> LLEAIAIALTAAHFGAPLLYYWRAKRWLKKPWDVAPDPTYRPRV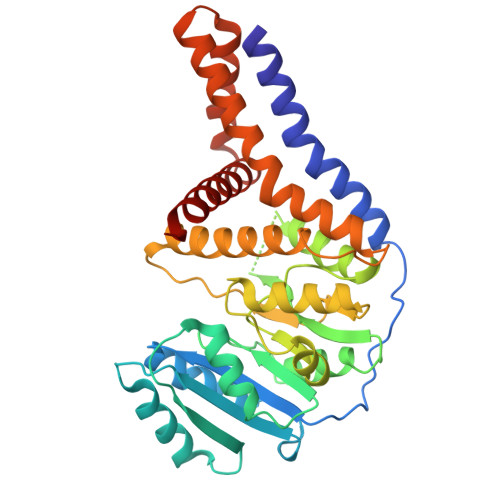TVIVPTYNEAPLIEEKLDNIYEQDYPRDKLEVVVVDSASTDGTPSAVRRWAETHPDLALTLVEETERRGKAHALNTALRHATGEIVVITDADALWPARDTLANAVKWLADPTVGAVSCVKRPAGPAGVEDSYRDFYNVLRVAESKAWATPIFHGELAAFKRELLERLGGFPTDVGADDSHTATKIAMMGYRAITPPDVVCVEAVPKRGYHAWRIRRAQHLVQHFAKAIRDGKAPPPFKPILHAEAYLHLANPWALPTAAAALAAAAAAGSLPAAALLATGAALALYKPYRTWTTMQAYLIAAAVKNLWDKE> NLFQ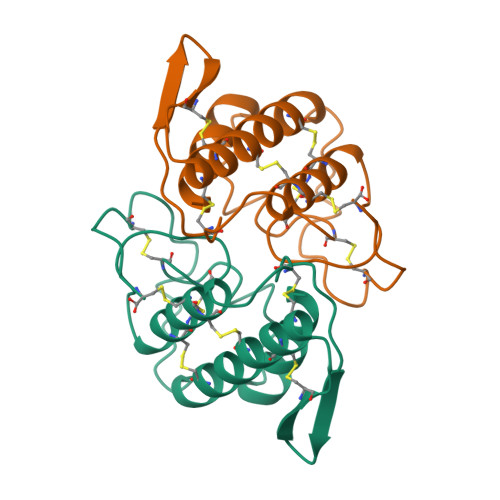FGDMILQKTGKEAVHSYAIYGCYCGWGGQGRAQDATDRCCFAQDCCYGRVNDCNPKTATYTYSFENGDIVCGDNDLCLRAVCECDRAAAICLGENVNTYDKNYEYYSISHCTEESEQC>GSSPVQSGFNNGTISNYMYFERRPDLLTKGTQDKAAAVKLKIENFYQSSVKYAIERNERRVELETELTSHNWSEERKSRQLSSLGKKESQFLRLRRTRLSLEDFHTVKVIGKGAFGEVRLVQKKDTGKIYAMKTLLKSEMYKKDQLAHVKAERDVLAGSDSPWVVSLYYSFQDAQYLYLIMEFLPGGDLMTMLIRWQLFTEDVTRFYMAECILAIETIHKLGFIHRAIKPDNILIDIRGHIKLSDFGLSTGFHKTHDSNYYKKLLQQDEATNGISKPGTYNANTTDTANKRQTMVVDSISLTMSNRQQIQTWRKSRRLMAYSTVGTPDYIAPEIFLYQGYGQECDWWSLGAIMYECLIGWPPFCSETPQETYRKIMNFEQTLQFPDDIHISYEAEDLIRRLLTHADQRLGRHGGADEIKSHPFFRGVDWNTIRQVEAPYIPKLSSITDTRFFPTDELENVPDSPAMAQAAKQREQMTKQGGSAPVKEDLPFIGYEYSRFDYLTRKNAL[2x];>GSRNKHHSPKRHSQTSFPAQKSTPQSQQLTSTTPQSQQQEASERSESQQIMFLSEPFVRTALVKGSFKTIVQLPKYVDLGEWIALNVFEFFTNLNQFYGVVAEYVTPDAYPTMNAGPHTDYLWLDANNRQVSLPASQYIDLALTWINNKVNDKNLFPTKNGLPFPQQFSRDVQRIMVQMFRIFAHIYHHHFDKIVHLSLEAHWNSFFSHFISFAK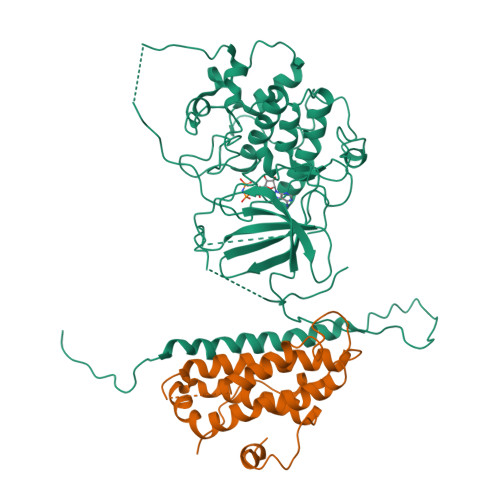EFKIIDRKEMAPLLPLIESFEKQGKIIYN[2x]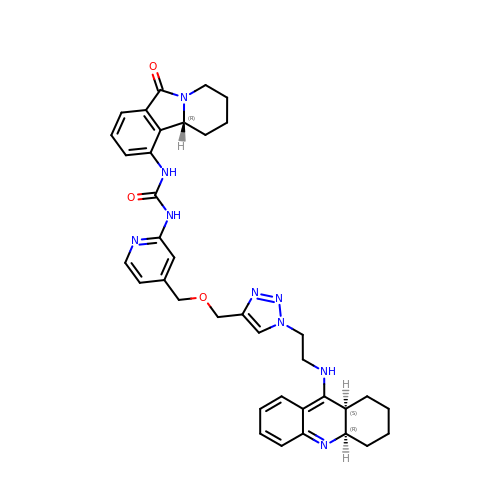1-[4-[[1-[2-(1,2,3,4,4~{a},9~{a}-hexahydroacridin-9-ylamino)ethyl]-1,2,3-triazol-4-yl]methoxymethyl]pyridin-2-yl]-3-[(10~{b}~{R})-6-oxidanylidene-2,3,4,10~{b}-tetrahydro-1~{H}-pyrido[2,1-a]isoindol-10-yl]urea | C37 H41 N9 O3 | UJAHYENXDKLQNE-TXKQGMEVSA-N> MSQVNTSQGPVAQGRQRRLSSLSEFNDPFSNAEVYYGPPTDPRKQKQAKPAKINRTRTMSVFDNVSPFKKTGFGKLQQTRRGSEDDTYSSSQGNRRFFIEDVDKTLNELLAAEDTDKNYQITIEDTGPKVLKVGTANSYGYKHINIRGTYMLSNLLQELTIAKSFGRHQIFLDEARINENPVNRLSRLINTQFWNSLTRRVDLNNVGEIAKDTKIDTPGAKNPRIYVPYDCPEQYEFYVQASQMHPSLKLEVEYLPKKITAEYVKSVNDTPGLLALAMEEHFNPSTGEKTLIGYPYAVPGGRFNELYGWDSYMMALGLLEANKTDVARGMVEHFIFEINHYGKILNANRSYYLCRSQPPFLTEMALVVFKKLGGRSNPDAVDLLKRAFQASIKEYKTVWTAS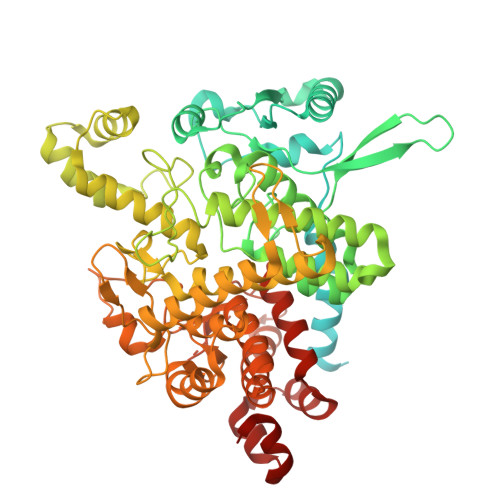PRLDPETGLSRYHPNGLGIPPETESDHFDTVLLPYASKHGVTLDEFKQLYNDGKIKEPKLDEFFLHDRGVRESGHDTTYRFEGVCAYLATIDLNSLLYKYEIDIADFIKEFCDDKYEDPLDHSITTSAMWKEMAKIRQEKITKYMWDDESGFFFDYNTKIKHRTSYESATTFWALWAGLATKEQAQKMVEKALPKLEMLGGLAACTERSRGPISISRPIRQWDYPFGWAPHQILAWEGLRSYGYLTVTNRLAYRWLFMMTKAFVDYNGIVVEKYDVTRGTDPHRVEAEYGNQGADFKGAATEGFGWVNASYILGLKYMNSHARRALGACIPPISFFSSLRPQERNLYGL> LLSLCKIPTFLGNLDSNKKRIPYFSATNSTPATPLVTYQVTLSCSCMANSMLAAVARNFNQYRGSLNYLFVFTGSAMTKGKFLISYTPPGAGEPKTLDQAMQATYAIWDLGLNSSYNFTVPFISPTHYRQTSYNTPTITSVDGWLTVWQLTPLTYPLGVPNDS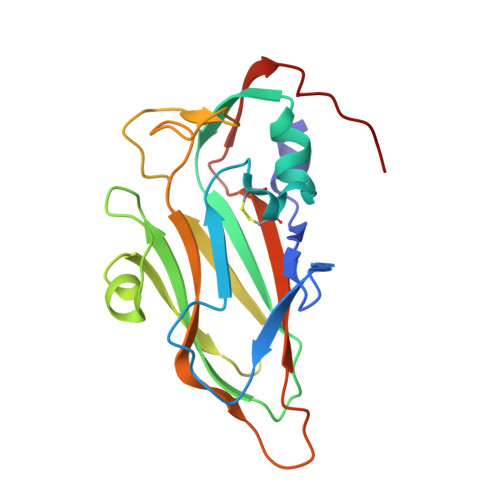HILTLVSGGDDFTLRMPVTFTKYVPQ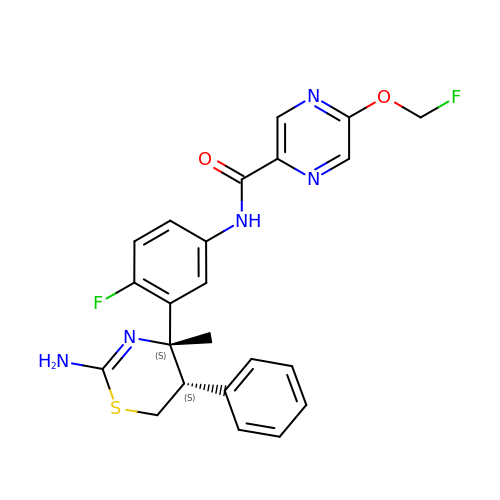N-[3-[(4S,5S)-2-azanyl-4-methyl-5-phenyl-5,6-dihydro-1,3-thiazin-4-yl]-4-fluoranyl-phenyl]-5-(fluoranylmethoxy)pyrazine-2-carboxamide | C23 H21 F2 N5 O2 S | BCDWEYSMCDBNJS-GAJHUEQPSA-N>GPLGSMRKQALHPRTAVINKAQKNQSKRARSDALLWLAANFPEAFDNSLRIRPLKIGIMSDILQHAEKAEQVGVSKSKLREAVVLFTRRLDYLACLKAREVRIDLHGNPVAEVTEEEAENASMKIKKRVEK[9x]

The ProQ/FinO family of RNA binding proteins mediate sRNA-directed gene regulation throughout gram-negative bacteria. The RocC/RocR system regulates competence, a specialized physiological state involving the coordinated expression of multiple genes which allows the bacteria to uptake environmental DNA and integrate it into its chromosome (i.e., natural transformation). RocC binds and stabilizes RocR, which in turn binds and represses a series of mRNA targets that encode components of the DNA uptake system.

Deletion of the N-terminal 13 residues, which are disordered in our structures, did not impact RNA-binding affinity or transformation repression. Furthermore, we tested the binding affinity of a RocC construct containing an additional C-terminal predicted helical region (RocC1-137). This construct had the same binding affinity as 1–126, indicating that this additional region does not play a significant role in RNA binding.>[4x]SMTTNGADPLGRFSALTREWFTTAFAAPTPAQADAWSAISEGNNTLVIAPTGSGKTLAAFLWAIDRLADPAREPSQGTQVLYVSPLKALAVDVERNLRTPLTGITRVAERHGLPAPSITVGVRSGDTPPNQRRAMIANPPDVLITTPESLFLMLTSAARETLTSVRTVIVDEVHAVAATKRGAHLALSLERLDQLLDTPAQRIGLSATVRPPEEVARFLSGQAPTTIVCPPAAKTFDLSVQVPVPDMANLDNNSIWPDVEERIVDLVEAHNSSIVFANSRRLAERLTSRLNEIHAERSGIELPAGPNPEVGGGAPAHLMGSGQANGAPPLLARAHHGSVSKEQRAQVEDDLKSGRLRAVVATSSLELGIDMGAVDLVIQVEAPPSVASGLQRVGRAGHQVGEISQGVLFPKHRTDLIGCAVTVQRMQTGDIETLRVPANPLDVLAQHTVAVAALEPVDADAWFDAVRRSAPFATLPRSAFEATLDLLSGKYPSTEFAELRPRLVYDRDTGTLTARPGAQRLAVTSGGAIPDRGMFTVYLASETEKPSRVGELDEEMVYESRPGDVISLGATSWRITEITHDRVLVIPAPGQPARLPFWRGDSVGRPAELGAAVGAFTGELASLDRKAFDKRCQKMGFAGYATDNLHQLLREQREATGVVPSDTTFVVERFRDELGDWRVILHSPYGLRVHGPLALAVGRRLRERYGIDEKPTASDDGIIVRLPDSGDTPPGADLFVFDADEIEPIVTAEVGGSALFASRFRECAARALLLPRRHPGKRSPLWHQRQRAAQLLDIARKYPDFPIVLEAVRECLQDVYDVPALIELMHKIAQRRLRIVEVETATPSPFAASLLFGYVGAFMYEGDSPLAERRAAALALDTVLLSELLGRVELRELLDPAVVASTSAQLQHLTPERAARDAEGVADLLRLLGPLTEADIAQRCTAD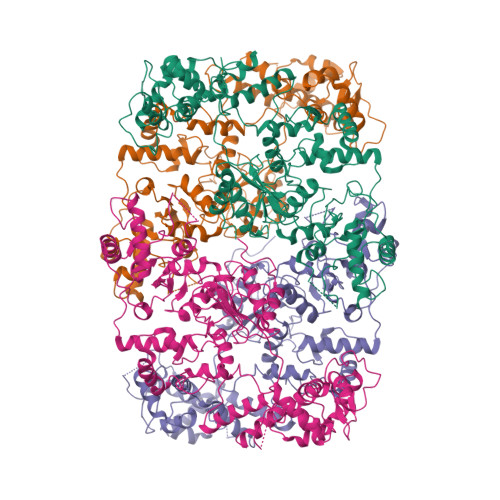NIGAWLDGLHAAKRALPVTYAGQTWWAAVEDIGLLRDGIGVPVPVGVPAAFTESASDPLGDLIGRYARTRGPFTTEQTAARFGLGVRVASDVLSRMAVDGRLIRGEFAADLSGEQWCDAQVLKILRRRSLAALRAQVEPVSTDAYARFLPSWQHVGSTNTTGVDGLATVIEQLAGVPIPASAVESLVFPQRVRDYQPAMLDELLASGEVMWSGAGQIGNGDGWVAFHLADTAPLTLTHGAEIEFTDTHRVILETLGHGGAYFFRQLTDGTVEGTAGQELKQALWELIWAGWVTGDTFAPVRAVLSGPRRSGAPAHRQRQRPPRLSRYSVAHAQTRGTDPTVSGRWSALPAAEPDSTVRAHFQAELLLGRHGVLTKGAVGAEGVPGGFATLYKVLSAFEDAGRCQRGYFVESLGGAQFAVASTVDRLRSYLDNVDPERPEYHAVVLAATDPANPYGAALGWPTDSEAHRPGRKAGALVALVDGRLVWFLERGGRSLLSFGADADAQRAAAGALTDLVSAGRIPSLLVERINGVAVLDPDVDAERAVVQDALLGAGLSRTPRGLRLR>MIHLRPDSTAYARSAAVSANPAVGGYVTPDNTVLEGQNPSALVQAMQKPVASVTDSFKATLSESIGAKALRGVEYASIPTEAGFEPSKALGDSVSQYTADELEFLSDARSSAELAQRRSQVQDTRNNYDAMGQNMLTTVAASMLDVDMVIGGGVGALSKVSRATRLAVGLSANAALLGTASYGGTITPLDVVGTSVGIAMSAIPGIRKVAKAEQVQQGAVRGGVNAAEDAAGTVVPPKDVTVPPVREVPEVQPIKTVADEDYPKIDIDTYSNKEHIEVGRTGGAKTGSLKTTVQNAVLAVTALGDDLPEGVRALGRALGASLEADADVPVVFRSRTGANAQARSAVITEAETGATRAEIFNPAVGGTLSDHVRGMSTYEKTILLHEAAHAKTGRSIRAVESGAVSDGVVYEAVQRIKEIQWYVKANVELPPLGKGAKYNVDYGLSDTHEFISQLFNSEHFRDALRSVKMPGSDGTLLSNLMKRVVTLFTGKAPEGNAFDATLQAFDNLLSQPTTPADVFLNAPKATPDLQSKVLQAPNVIEMNNKVMGALNRNFSLYERLKSFGYKASTLADQLVVDATGTEANSAAHHARAAHLASNVSIVQVDDAFRQALSADWPLVQRLRHPVLYREAQRDLSQKVYQQLAENHDRFLKGQSIQPSNDPRVNSMVDAFVNSNWAKDELARVKGAGINGADAVRESPYYLPRQHSGNKLNDFMRNNRQVTKDDIVGMYTEQFSRMFQQNGITPETARKLGAKMFDNMQDQAAHVQGYRQSIAGMSYDDIENTLEALGASDPTITAFLDAVKGSGEQANKVRNLRGRAEFDMTAQYTTKSGDMISPSMFVNNDVMGLMEGYSRRMSGRVGLAKAGFPDLRDAVKAIDEAAAEAQDPAAALHAFDNTMNQILGYPTGEDVPDILRSASIIGGALNLANSGIYQLADMSLMLQQFGITKTLKAFGSTAFGRNAMDVAKSAEFGSRLQDVIEARHVLSGKYRSVLTHLEDNRDIGSLGVAHRYVQQMGQGTRFVNGMEFIRRGQAKLVSGLIADTVDDAIAGNASAVTAMERFGLNQQLLDELRKATAANPDMRKWPDSVRMDIEAVTHNMADSIVLENRLGEIPAWMQFSSVGKVILPYMTFVAGAWNKILRRTAKLDGATGVAIALAYQMPLVTLSSATSIAISGKPVTPESVAQRALVQVPMMSWAGFAVDFWANGASNNLAALALVDRMHAAMSSIASGETNPESLIKAVPFLSILPGMRLMGASLADDDE[4x];>MPVRQPTQGGVQVPGLTGYQSAGVAQPVYRAPQEEAQGVSQFWQNLLPASVKTAQAAQQTASAKGYLEGQQDSQQGREKQVRNFFTKEAYEQGYNSASVNSALASFQLGLQNTAQQYVNSGKTPEEFNVHVQQQTNQLLQEAGAQGLNLNDKDWQAWLGSVEHSRNTANASYQDLNLKRAAVLQEQSWGARGNAAIADFVTAQQSGDTEQALQNVNSFISSVTHDDSITAENKIKYTSQFVVNAFANANSTGDMQALTGYVQSLSEFKNMPTDVQTQIMGSAQQYYQQRASDESVQLYEYNSRVNSVTDYKTLNEAYPMAQYIGTVMQAVQQKKLSPGTGYGMVDAESQRRLKMQKAEQGQLAYTNGVTISDIAAGTGESLDKVKGELTKMYATIGQGYSGGGLQLMQRGLKSGAQDITGVGIEMMQQDAQSLSGIDWRNLKTDADGKPLYPAAVVGSLGNLQAAYQSALAAGNQVQANQLLSGLPDPVVYGIRQNVDARDLADVVGKRAQDIASGKVLALPANMPADVSITQADVTAGIFDLGLGKDARNRNMLGIQSWVFTSDADEKAAQARVSQVNSAMNNEYVYNQQRGSLPALVGDDLKSWLMGKVASRTVRVKDGTDNGALLVLPEVGDKQKVFGSTDNGIIESALTESVTNFKKQYPQATTVQMDYDPLTQELIFQGVNAENQLGTTRASIPAADFRNTVRGVQNTLTQNGSGTTQGNLNVPGAGFVSFNAGNSFGIQKNVVMGAVNQLVSYEGYTPSKGFSVLGVHPTTGAKLNEDKYVKQATDTPQVAADKFNMYLNDKVYPLVMPKMEQYKNLPGYIQNNIYNALVETTYHSGNSDVFDKYIQTALYGNVQEIPTFKDTPLFKDAGAGSRRNVDRYQLLGSLVTYRTNNPNLSK[8x];>MIWMFAAAAAQMIQGGLQYAQDAKNQRRQNKADQKYNEAVRSASARQITEINTQRSVSRAQTAQALDAARRQGAGESSARNLQAAATDTMGASVEQNLQEVGVQLAAAEGNLMQNAELTELSLDSSVMNTVDQARNSIRELSNPLGTDWAATGSAVGQIGTSMVANKLGGQGWFGGNSGTQQPAPISQAAPPTRSNNLSTRLNV[8x]

Podophages that infect gram-negative bacteria, such as Pectobacterium pathogen ΦM1, encode tail assemblies too short to extend across the complex gram-negative cell wall. To overcome this, podophages encode a large protein complex (ejectosome) packaged inside the viral capsid and correspondingly ejected during infection to form a transient channel that spans the periplasmic space. Here, we report a near-complete atomic model of the bacteriophage ΦM1.

Here, we describe the ejectosome of bacteriophage ΦM1 to a resolution of 3.32 Å by single-particle cryo-electron microscopy (cryo-EM). Similar to that of bacteriophage T7, the ΦM1 ejectosome is encoded as a three-protein mega complex composed of TEP, OEP, and EP3 oligomers arranged coaxially within the phage capsid. The capsid houses a large ejectosome complex composed of TEPs (, gp48), octameric ejection proteins (OEPs, gp49), and ejection protein 3 (EP3, gp50) arranged axially above the crown of the portal complex (gp35). The EP3 octamer adapts the locally 8-fold symmetric interface of the ejectosome to the 12-fold symmetric crown of the portal by intercalating the EP3 helix α-2 between the crown domains of adjacent portal monomers, forming contacts with the C-terminal portal helix. Through a combination of BLASTP and DALI homology searches, putative enzymatic domains were identified in the ejectosome, specifically a lysozyme-like domain within the OEP (Gly718–Ser903) and an endolysin/exotransglycosidase-like domain within the TEP (Asp268–Asp528). Viral lysozymes and exotransglycosidases can digest peptidoglycan, suggesting that these domains may degrade local peptidoglycan surrounding the periplasmic channel once ejected from the phage particle during infection. The T7 ejectosome adapts by slipping around a pedestal-like barrel created by the portal crown, whereas the ΦM1 ejectosome adapts on top of the portal through intercalating helices which form an analogous barrel. In T7, the TEP consists of an N-terminal LTase followed by the hub domain. However, in ΦM1, the helical hoop and endolysin-like domain are inserted into the hub domain. Further, the ΦM1 OEP has an additional lysozyme-like domain which T7 lacks.Central to this ability are non‐canonical covalent intramolecular crosslinks between protein side chains forming isopeptide, thioester, and ester bonds that impart remarkable stability enhancement to single adhesin protein domains or are involved directly in covalent adhesion to host cells (Alegre‐Cebollada et al. 2010; Kang et al. 2007; Kang and Baker 2009; Kwon et al. 2014; Lei et al. 2021; Miller et al. 2018; Pointon et al. 2010; Walden et al. 2015). The autocalytic machinery of ester bond crosslinking, as first exemplified in the Clostridium perfringens adhesin Cpe0147, shows three residues (D577/H572/T450) arranged in space to mimic the acid/base/nucleophile catalytic triad of a serine protease, with Q580 the equivalent of a substrate electrophile (Kwon et al. 2014; Schwarz‐Linek and Banfield 2014). Two buried and protonated acids, D480 and E547, act like the oxyanion site of a serine protease, polarizing the carbonyl bond of Q580 side chain to increase its electrophilic potential and reactivity, and potentially stabilizing a high‐energy tetrahedral intermediate. In the proposed mechanism, H572 abstracts a proton from T450 Oγ1, which then effects nucleophilic attack on the Q580 Cδ with the loss of the side chain amino group as ammonia—the final state is the equivalent of the acyl‐intermediate of a serine protease mechanism, but without the potential to hydrolyze it is essentially trapped.

The T450C protein is found predominantly as non‐crosslinked and disulfide crosslinked species under non‐reducing SDS‐PAGE —this scenario is detailed below in the SEC‐MALLS and X‐ray crystallography results. Only a very small proportion of T450C protein forms the smallest hydrodynamic radius, crosslinked species eluting similarly to the wild‐type protein at ~12.5 mL and with a thioester crosslink confirmed by mass spectrometry. A close inspection of the mutation site shows no thioester crosslink with the C450 thiol group sequestered in the pocket otherwise occupied by the methyl group of the wild‐type T450. The reactive sidechain of Q580 forms hydrogen bonds through both Oε1 and Nε2 atoms with the protonated buried acid, D480. The position of E547 is unchanged compared to the wild type, pointing away from the ester bond position and making a hydrogen bond with D480. A wild‐type, non‐crosslinked model was produced from the T450C structure. Geometric analysis following the method of Du et al. formulated for serine protease characterization gives an attack distance, d attack, of 2.65 Å measured between nucleophile Oγ and electrophile target atom Cδ (Du et al. 2025). The attack angles α attack and φ attack are calculated at 104° and 89°, respectively. In this model, the close approach (2.65 Å) of nucleophile threonine Oγ and electrophile glutamine Cδ, and the perpendicular relative orientation of the side chains, are consistent with the geometric arrangement observed by Du et al. within 1000+ serine proteases (Du et al. 2025).

>[2x]GAMDPEFNLPEVKDGTLRCTVIADGVNGSSEKEALVSFENSKDGVDVKDTINYEGLVANQNYTLTGTLMHVKADGSLEEIATKTTNVTAGENGNGTWGLDFGNQKLQVGEKYVVFENAESVENLIDTDKDYNLDTKQVVKHEDKNDKAQTLVVEKP>SGVRPESGVGPESGVGPEAGVGPEAGVGPESGVGPEAGVGPEAGVGPESGVGPESGVGPEAGVRPEAGVRPEAGAGTDTETEEEIEEVVGDEEALAYLNETVIDPKLIALLDDFGVSRSGRKAISYIQGNLTSDVIYDRLNKLGADVVIEKIIKPTVSLLKTKGEALKIIEDPTNEGVKTRLQNMCKRYDGLVKGIGYDFFHGSIGTDRFAQAVVYYAPRFRKFKEIVKNPRVMDDIYGWLDADDRATINEIGKIVINATYDKDKFNNVLNSVGVYYVVRMIDIYRGVK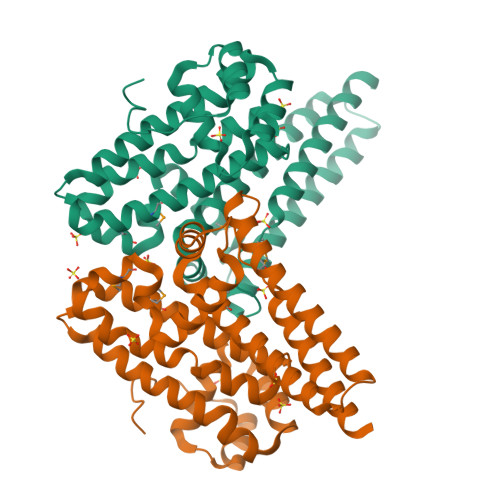IEHDEALNAITTVPDGVVKQDLQARLNRFKGEYYSNIRGTFKGFTDGLHFQIMTDGDKYRNYFIILKFDAQAARVAKARGATGSGS[2x]Trx is a small redox-active protein (∼12 kDa), which has a conserved CxxC catalytic site that undergoes reversible oxidation/reduction of both cysteine residues whereas TR is a member of the flavoprotein family of pyridine nucleotide disulfide oxidoreductases and functions in a homodimeric form. Within each TR monomer, reducing equivalents are transferred to Trx from NADPH via a tightly TR-bound flavin adenine dinucleotide (FAD) and a redox-active disulfide (CxxC motif). A third TR named DvTRi (i for isolated) was identified in Desulfovibrio vulgaris Hildenborough (DvH). Enzymatic and structural characterization of DvTRi clearly shows that NAD(P)H does not serve as electron donor for the FAD while DvTrx1 was identified as the substrate.

The crystal structure of oxidized DvTRi was solved at 2.0 Å resolution, with one physiological homodimer per asymmetric unit. Each monomer is composed of a FAD-binding domain (residues 1–109 and 231–309) and a pseudo NADPH-binding domain (residues 119–225) linked by an interdomain hinge region (residues 110–118 and 226–230). The FAD protein environment is well conserved in DvTRi with a similar binding mode, through a network of supramolecular interaction involving structural water molecules and the conserved binding-motifs GxGxxG, ATG and GxFAAGD. The electron density of FAD is well defined with an occupancy close to 1 and the isoalloxazine ring of FAD is planar. In the pseudo NADPH-binding domain, the signature motifs VxxxHRRDxxRA and GGGxxAxE required for NADPH binding are replaced with the VxxxTQGKxxSI and the GEGxxAxN motifs, respectively. The only basic amino acid in the motif is lysine 174, which is well superposed with arginine 176 in EcTrxB. However, it is not sufficient to stabilize the phosphate group of NADPH since its binding requires seven salt bridges with three arginines in EcTrxR. The absence of crucial residues in DvTRi required for the binding of NADPH excludes the possibility for the enzyme to physiologically use this reductant, which is in complete agreement with our biochemical data. Whatever the crystallization conditions were, the different structures we solved from crystals 1 or 2 showed an unexpected unique conformation of DvTRi, that differs from both FO and FR conformations observed in EcTrxB structures. The structure revealed that the two active-site cysteines (the CxxC motif) are far away from FAD.

>[2x]METRPLVIIGAGPAGLSAAVYTARAGIPTLVFGSAPKVAGDYDIDNYFGFDETITGRELIERGRRQAERFGAVLRDDRILGLHHGDDGGFRITTEAGETAACAIILATGVSRVRPGISNIADYEGKGVSYCVSCDGFFYRGLRVKVLGEGVFAANQALELLHYTPHVSICTQGKAASITPEFMTRLDEAGIAVDDRKIASLEGTPALSVLRYEDGSTEEAQGLFIAMGEASSLDFAYTLGVERNGVFLGADSDQRTNIPGVFAAGDCTGGFLQIAVAVGEGAKAARAAISYIKEECPFATSRRNTTTES> MRQVWFSWIVGLFLCFFNVSSAKEPCPPENLQLTPRALVGKWYLRTTSPD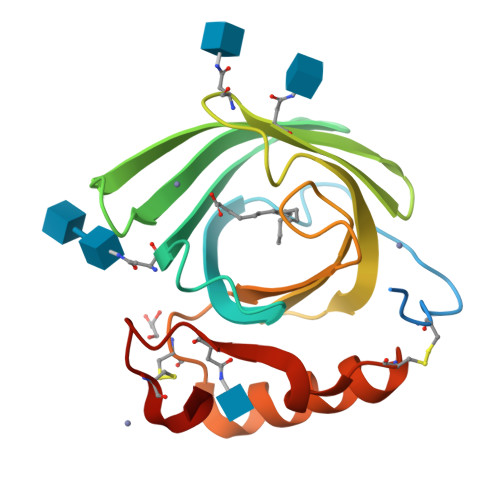IFKQVSNITEFYSAHGNDYYGTVTDYSPEYGLEAHRVNLTVSGRTLKFYMNDTHEYDSEYEILAVDKDYFIFYGHPPAAPSGLALIHYRQSCPKEDIIKRVKKSLKNVCLDYKYFGNDTSVHCRYLE>[6x]MLYVYMDGEFVPENEAKVSIFDHGFLYGDGVFEGIRAYNGRVFRLKEHIDRLYDSAKAIDLEIPITKEEFMEIILETLRKNNLRDAYIRPIVTRGIGDLGLDPRKCQNPSIIVITKPWGKLYGDLYEKGLTAITV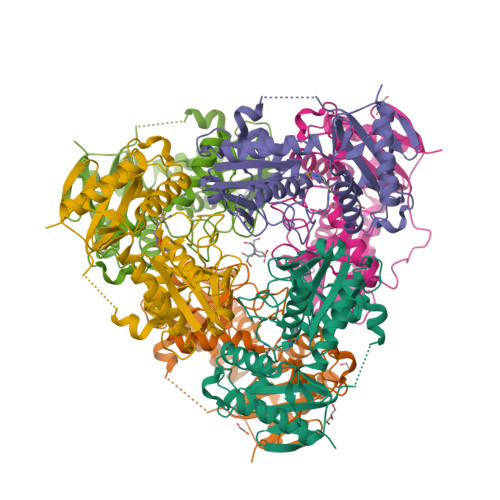AVRRNSFDALPPNIKSLNYLNNILAKIEANAKGGDEAIFLDRNGYVSEGSGDNIFVVKNGAITTPPTINNLRGITREAVIEIINRLGIPFKETNIGLYDLYTADEVFVTGTAAEIAPIVVIDGRKIGDGKPGEITRKLMEEFSKLTESEGVPIYE> STQDADRTLKRLQLQMDNLESRVALECKEAFAELQTDINELTNHMDGVQIPFLDYRTYAVRVLFPGIEAHPVLKELDTPPNVEKALRLFGQLLHSRAFLLTFIHTLEAQSSFSMRDRGTVASLTMVALQSRLDYATGLLKQLLADLIEKNLESKNHPKLLLRRTESVAEKMLTNWFTFLLHKFLKECAGEPLFLLYCAIKQQMEKGPIDAITGEARYSLSEDKLIRQQIDYKTLTLHCVCPESEGSAQVPVKVLNCDSITQAKDKLLDTVYKGIPYSQRPKAEDMDLEWRQGRMARIILQDEDITTKIECDWKRVNSLAHYQVTDGSLVALVPKQVSAYNMANSFTFTRSLSRYESLLRAASSPDSLRSRAPMLTPDQEAGTKLWHLVRNHDHTDHREGDRGSKMVSEIYLTRLLATKGTLQKFVDDLFETVFSTAHRGSALPLAIKYMFDFLDEQADQRQISDPDVRHTWKSNCLPLRFWVNVIKNPQFVF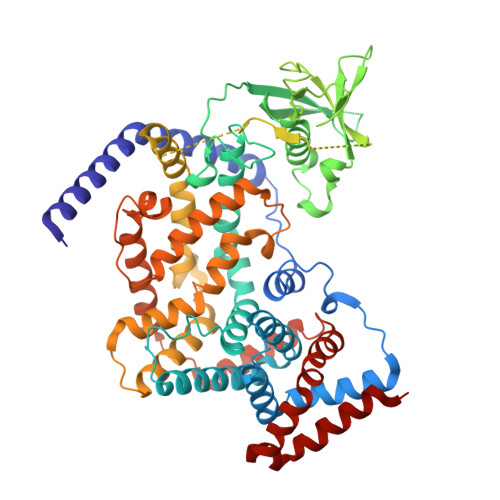DIHKNSITDACLSVVAQTFMDSCSTSEHRLGKDSPSNKLLYAKDIPNYKSWVERYYRDIAKMASISDQDMDAYLVEQSRLHANDFNVLSALSELYFYVTKYRQEILTSLDRDASCRKHKLRQKLEQIITLVSSSS> MRGSHHHHHHGSMPVAGSELPRRPLPPAAQERDAEPRPPHGELQYLGQIQHILRCGVRKDDRTGTGTLSVFGMQARYSLRDEFPLLTTKRVFWKGVLEELLWFIKGSTNAKELSSKGVKIWDANGSRDFLDSLGFSTREEGDLGPVYGFQWRHFGAEYRDMESDYSGQGVDQLQRVIDTIKTNPDDRRIIMCAWNPRDLPLMALPPCHALCQFYVVNSELSCQLYQRSGDMGLGVPFNIASYALLTYMIAHITG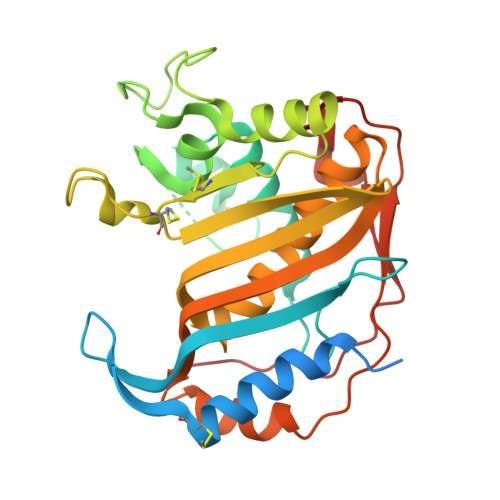LKPGDFIHTLGDAHIYLNHIEPLKIQLQREPRPFPKLRILRKVEKIDDFKAEDFQIEGYNPHPTIKMEMAV(3aR,5R,5aR,8R,8aR,9aR)-5-methanoyl-8,9a-dimethyl-2-propan-2-yl-3,3a,4,5,5a,6,7,8,8a,9-decahydrocyclopenta[g]azulene-1-carboxylic acid | C20 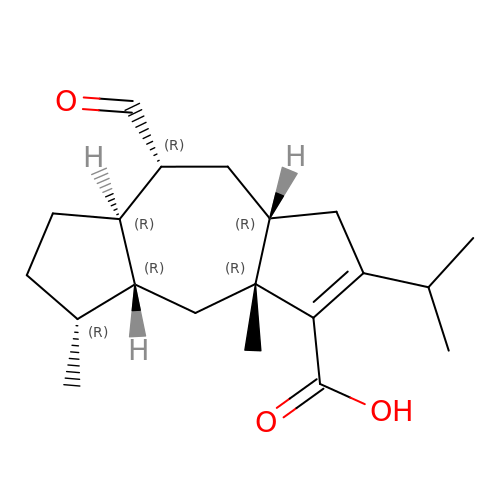H30 O3 | WHZYJBLNTIYKIO-JXWLXEMXSA-N[[(2~{R},3~{S},4~{R},5~{R})-5-(6-aminopurin-9-yl)-4-oxidanyl-3-phosphonooxy-oxolan-2-yl]methoxy-oxidanyl-phosphoryl] [(3~{R})-2,2-dimethyl-4-[[3-[2-[(1~{R})-2-(1-methylpyridin-4-yl)-1-naphthalen-1-yl-ethyl]sulfanylethylamino]-3-oxidanylidene-propyl]amino]-3-oxidanyl-4-oxidanylidene-butyl] hydrogen phosphate | 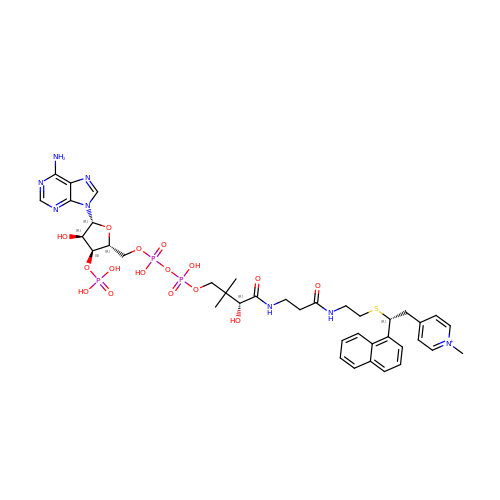C39 H52 N8 O16 P3 S | OYNQMIGIWWZLSR-UAMJECFJSA-O> AGVMTGAKFTQIQFGMTRQQVLDIAGAENCETGGSFGDSIHCRGHAAGDYYAYATFGFTSAAADAKVDSKSQWKLLAPSAPTLTLAKFNQVTVGMTRAQVLATVGQGSCTTWSEYYPAYPSTAGVTLSL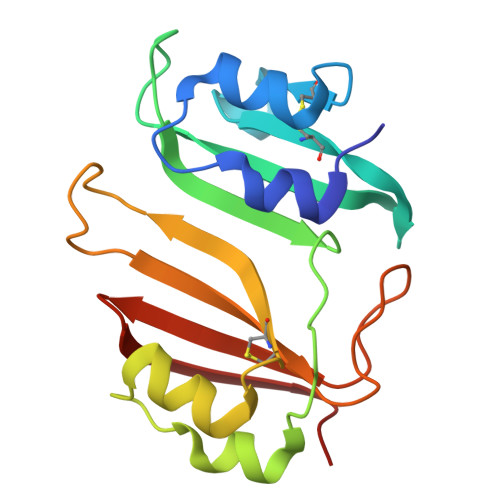SCFDVDGYSSTGFYRGSAHLWFTDGVLQGKRQWDLV4-(dimethylamino)-1-{4-[4-(4-{[4-(pyrrolidin-1-yl)pyridinium-1-yl]methyl}phenyl)butyl]benzyl}pyridinium 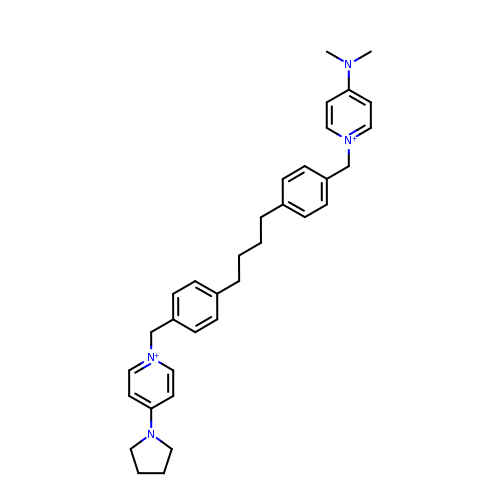| C34 H42 N4 | OXXBKOUHROTSGV-UHFFFAOYSA-N> MGRLLRLEVENFKSYRGHQIIGPFEDFTSIIGPNGAGKSNLMDAISFVLGVKSSHLRSTNVKELIYRGKILQRDNTDFTDSSNPTTAYVKLMYELDNGEQREYKRAITPSGATEYKIDEEIVTFSEYCGSLQKENILVRARNFLVFQGDVETIASQSPLELSKLVEQISGSLEYKSEYDKSKDEQDKAVNLSAHSFNKKRGINAELRQYQEQKTEAERYQSQKEKRDSAQLVYLLWKLFHLEKSISSNMAEVTRLKADSIQLIERRDENTKEIEKLKEKEGSIRRNLLAFDRKVRKQEKLIASKRPELISIAEKALESKSNLRKIQRKAAEIEKDYSDQASTLQVLENQLTSLSAAEKEFLKDMQEKEQLKGLRLLPEDKEEYEGLRSEADKLNSNLLFKLQTLNRNIKVTSQSKDSLTSIVGDLESKIKSLHESVSSLDTERADLLAKINEKIESLELEKHDQQKKRLTYSELFHKTQELNEELQSCLQKILEASADRNESKQDAKKREALYALKRIYPEVKGRIIDLCTPTQKKYESAIAAALGKNFDAIVVETQAVAKECIDYIKEQRIGIMTFFPMDTIAASPVNQKFRGTHKGARLAIDVLNFESEYERVMISAVGNTLICDSMTVARDLSYNKRLNAKTVTLEGTVIHKTGLITGGSSNNRSAKHWDDHDFDLLTQTKDRLMHQIGEIEYQKSSCVITESDTVKLHSLESEISLLKDKYTVVSRSVEDKKKEIGHYESLIKEKQPHLSELEMELRNFVKSRDELQIQVEKVEEKIFSGFCKRIGISDIHTYDEIHRTFTQSFTQKQLEFTKQKSLLENRISFEKQRVSDTRLRLERMHKFIEKDQESIDNYEQNREALESEVATAEAELELLKEDFASENSKTEKILLAASEKKLVGKRLVSELTKLSGNITLLESEIDRYVSEWHAILRKCKLEDIDVPLREGSLTSIPIDDVSNSGDITMGEEPSEPVINFEKFGVEVDYDELDEELRNDGSESMASVLQEKLREYSEELDQMSPNLRAIERLETVETRLAKLDEEFAAARKAAKNAKERFNAVKQKRLQKFQAAFSHISEQIDPIYKELTKSPAFPLGGTAYLTLDDLDEPYLGGIKFHAMPPMKRFRDMDQLSGGEKTMAALALLFAIHSYQPSPFFVLDEIDAALDQTNVTKIANYIRQHASSGFQFVVISLKNQLFSKSEALVGIYRDQQENSSRTLSINLEGYVE;> MFYSEAILSKKGPLAKVWLAAHWEKKLSKVQTLHTSIEQSVHAIVTEETAPMALRLSGQLMLGVVRIYSRKARYLLEDCTEALMRLKMSFQPGQVDMIEPATALQSLKGKDAVTQSANLTLPETITEFDLLVPDSTFDFQWSQLLRTPSRSSNTLELHSLPISSSPSFPSSQLSIEAGRNAQVESGFSLGESFAHVGNDMQFHLPISNSGAATPRSVHSDNQSQISIEVGRDAPAAAATDLSGIIGPQMTKSPASSVTHFSTPSMLPIGGTSLDDELLAPVDDLNLDLGLDDLLGDEQGANAPAIEADEQAETSSIHLPSDIMEDDSSRPAAAGVEEGQVVESATAPQQEKINPQKTVRRQRAIIDPVTELSSKQMKKQLADTSSITSPLCLNTSSIVFNATVNFTRNGKFNTSIFSSNLNPKVNELLQADFKQAILRKRKNESPEEVEPAKHQRTDTSTENQETAEVLDPEEIAAAELANITEAAIATLPQETVVQPEGEAPELGSPMGFPVTALESADDSLFDAPPVMLDEADLLGSERLDSSVSEALPSSQTAKDSLRNKWDPYTEGEKVSFQTLSAGCNREEAVQLFFDVLVLATKDVISVKQDVAIQNEITLTAKRGMLLSSL;> MYITKIVIQGFKSYKDYTVIEPLSPHHNVIVGRNGSGKSNFFAAIRFVLSDAYTHLSREERQALLHEGPGATVMSAYVEVTFANADNRFPTGKSEVVLRRTIGLKKDEYSLDKKTVSKTEVINLLESAGFSRSNPYYIVPQGRVTSLTNAKDSERLELLKEVAGTQIYENRRAESNKIMDETIQKSEKIDELLQYIEERLRELEEEKNDLAVYHKKDNERRCLEYAIYSREHDEINSVLDALEQDRIAALERNDDDSGAFIQREERIERIKAEITELNHSLELLRVEKQQNDEDYTNIMKSKVALELQSSQLSRQIEFSKKDESSKLNILSELESKISEKENELSEILPKYNAIVSEADDLNKRIMLLKNQKQSLLDKQSRTSQFTTKKERDEWIRNQLLQINRNINSTKENSDYLKTEYDEMENELKAKLSRKKEIEISLESQGDRMSQLLANITSINERKENLTDKRKSLWREEAKLKSSIENVKDDLSRSEKALGTTMDRNTSNGIRAVKDIAERLKLEGYYGPLCELFKVDNRFKVAVEATAGNSLFHIVVDNDETATQILDVIYKENAGRVTFMPLNKLRPKAVTYPDASDALPLIQYLEFDPKFDAAIKQVFSKTIVCPSIETASQYARSHQLNGITLSGDRSDKKGALTAGYRDYRNSRLDAIKNVKTYQIKFSDLQESLEKCRSEIESFDQKITACLDDLQKAQLSLKQFERDHIPLKDELVTITGETTDLQESMHHKSRMLELVVLELHTLEQQANDLKSELSSEMDELDPKDVEALKSLSGQIENLSHEFDAIIKERAHIEARKTALEYELNTNLYLRRNPLKAEIGSDNRIDESELNSVKRSLLKYENKLQIIKSSSSGLEEQMQRINSEISDKRNELESLEELQHEVATRIEQDAKINERNAAKRSLLLARKKECNEKIKSLGVLPEEAFIKYVSTSSNAIVKKLHKINEALKDYGSVNKKAYEQFNNFTKQRDSLLARREELRRSQESISELTTVLDQRKDEAIERTFKQVAKSFSEIFVKLVPAGRGELVMNRRSELSQSIEQDISMDIDTPSQKSSIDNYTGISIRVSFNSKDDEQLNINQLSGGQKSLCALTLIFAIQRCDPAPFNILDECDANLDAQYRSAIAAMVKEMSKTSQFICTTFRPEMVKVADNFYGVMFNHKVSTVESISKEEAMAFVEG;> MLFEMTPETFKKVNSSNRIIKGLQYTPLASSIPLENGLQNVLYPSSKFQNEPLQLNSEESSIMQRYVDMLNPGATFVNDSETFNFYKNALSAMITEPAMPAMRVNASPVLDQKVCNSDSLSELNDFTKSLIQPSMLMCEPKEKPDASSINTNRSSSDNGFLTPSSSPRSPSCSRVFNAVQLCSPKKSKDDITTPKKRLMEDTYSPRESPSKIQRLQDVLLKQLQDTRLLISQVIEAENSEDFSSNSLFIKREDDDGKHISSHAIEKLYMALTKLSRLGACDKLLEEGSIILVKQILEKELKELPVACYSIINLHDSLTQFPNLDFILKTTALVLFIIFLVPSFKKLQNEESILHLLNILHSIFEYTVPEAIDNIVQSKTSDARTSEIQHLSVLLQKVANVLNILSKVAHEIPLSEAVVIRIVYLFPKVSTLDNSFKTKLPNCNSSSFDFLKAPLFQTLQYLFRLYPYQRDFIIEESLTNFSHLPTARSVSRTYRLSNGKSIQYYSTLFVRLIQSCSIQNLFDSEIVQSESKSTEALHSGNLTEHLKTVESILSKSRHEEYRIANHIVAYLLSRSLKQNKTESDNSFAILTKILLEDLLNMLSLPEWCGTETIIRQFAMNLVMTVTNDKQAVSSKNAALDLISLIVNKVLALFDLSLFEKHNIPAPTNFNDIISFIPSITRLNELSQVSFNHFYFLCKGDISLENILPYNYNKWFSFLLQLRKVCNDSEALKIIDNCIDKNMQKSQEGFQGPSPFKADENDEDIFIISLYHSSLFLNLKFFVSLIIGFLDSPQASLRTKCLRIINQMKTIPSILRTHPEVLAQIISKSNDQSAIVRDTVLDLLGTYIMAYRETIPQIYGCIISGISDPSTIVRKRAIKQLCEVYEATEDLNIRVDIASKLLTRSNDEEETISELSLEVLEKLWFSPASNELDCQKGYEQLTFLEKQKLRVQYFPILKLCAEPSTERHVLLVTSLKTMLTSK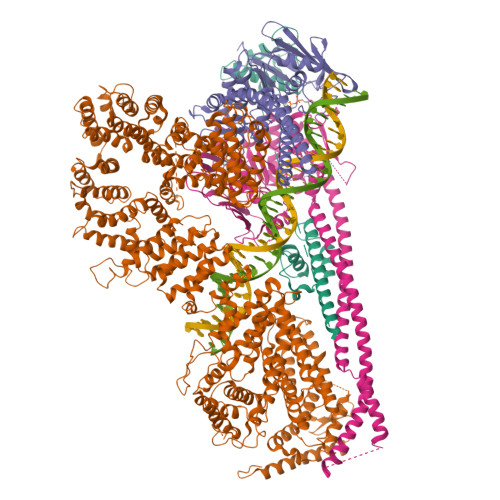EEINLSTLHTQIRLLLSCLFNQLIEVVTEDQVDESTKGILYEIMSTLFVFSRAFPFLFDLSYLHLLKPYLRSASTIEEQRFLYYVVAIFRQVLPFQKEISESFLRSLESVLLQRLTKAGTATLMEIVPCLCSLFTRLNDYERLKKIVVSCLKSLEEARHSENNFQKMVRLIDLIGLFSRYGDLNRINDDWKHSLDFISPECDDAYVILLGYFQKLLKDAKGQLRIHIIDNMSRICLRETSLFISPLMLSTLDMIIAENNVNEVSVLFKSFLELLAADEDLIFEADQKLSLKGKQNVQSNKSVDRDMLKGTKDKQWIEGVSASLMQHFLPCILDSCFSKNLRYSMLGIEILKCIIHQGLVNPRMCFSTIIALESNAIKETREVAILLHTELHRRHESLIDGLYAQSADLIFSLQKTEEYQTFKLGEFSPFQSAYTIVSADKSSKSRKKLIMQILKPLKLDGIDLPSFTEEKVSFVSFCCVCLAGIPYVSIEEPLMIISTVDSVLATIGPTITGWMKKLDHERFKILAGINLCNLIYLKRYIKYAFSISDSSRPIREKKPLTLLNRGYVDLITSDAKPDIVSKLVIKLFEEENILSGEDQVEGEQLTVV> ETLE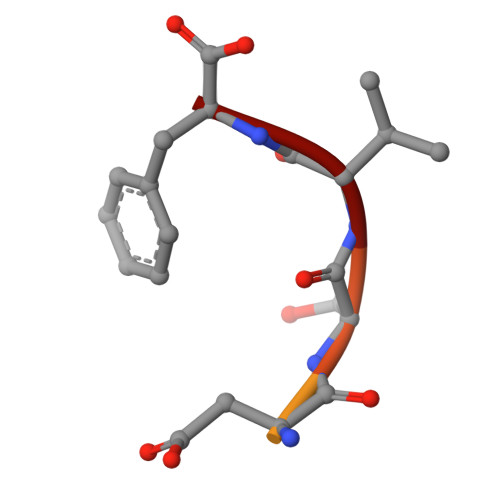DSVF>MEKSFVITDPRLPDNPIIFASDGFLELTEYSREEILGRNGRFLQGPETDQDIVSGATDAIRDQREITVQLINYTKSGKKFWNLLHLQPMRDQKGELQYFIGVQLDGEFIPNPLLG[2x]

By using a flavin transferase and carving a flavinylation motif in target proteins, we demonstrate that “dissociable” flavoproteins can be turned into covalent flavoproteins. Specifically, four different flavin mononucleotide-containing proteins were engineered to undergo covalent flavinylation: a light-oxygen-voltage domain protein, a mini singlet oxygen generator, a nitroreductase, and an old yellow enzyme-type ene reductase. The crystal structures of the designed covalent flavoproteins confirmed the designed threonyl-phosphate linkage. The elucidated crystal structures confirm that the covalent attachment does not significantly perturb the binding and microenvironment of the redox active part of the flavin cofactor.

Except for introducing a threonine residue at the respective positions, analogous to the engineering of PpSB1-LOV, the 6 residues before each site were also mutated to carve a recognition site for the flavin transferase into miniSOG as was done for the LOV protein (47-DAASGAT-53 for miniSOG-F1 and 51-DIVSGAT-57 for miniSOG-F2, respectively). To analyze the effects of covalent flavinylation on the structure of miniSOG, miniSOG-F2 was crystallized. The asymmetric unit contains two miniSOG-F2 domains. As observed for the LOV domain protein variants (vide supra), the structures of miniSOG-F2 and miniSOG are very similar (rms deviation on Cα atoms of 0.55 Å). The mutated residues of 51ATVQKIR57 to 51DIVSGAT57 are clearly visible in electron density. Electron density clearly confirms the introduced phosphoester bond between OG1 of Thr57 and the phosphate of FMN. The isoalloxazine group remains embedded at the same position in the protein. Only the angle of C5′–O5′–P is different and is bending toward Thr57. The phosphate group in miniSOG-F2 is further stabilized by the guanidino group of Arg41. The interaction in miniSOG with Arg57 is not observed, as in miniSOG-F2, it has been mutated to Thr57.>MMMASKDATSSVDGASGAGQLVPEVNASDPLAMDPVAGSSTAVATAGQVNPIDPWIINNFVQAPQGEFTISPNNTPGDVLFDLSLGPHLNPFLLHLSQMYNGWVGNMRVRIMLAGCAFTAGKIIVSCIPPGFGSHNLTIAQATLFPHVIADVRTLDPIEVPLEDVRNVLFHNNDRNQQTMRLVCMLYTPLRTCGGTGDSFVVAGRVMTCPSPDFNFLFLVPPTVEQKTRPFTLPNLPLSSLSNSRAPLPISSMGISPDNVQSVQFQNGRCTLDGRLVGTTPVSLSHVAKIRGTSNGTVINLTELDGTPFHPFEGPAPIGFPDLGGCDWHINMTQFGHSSQTQYDVDTTPDTFVPHLGSIQANGIGSGNYVGVLSWISPPSHPSGSQVDLWKIPNYGSSITEATHLAPSVYPPGFGEVLVFFMSKMPGPGAYNLPCLLPQEYISHLASEQAPTVGEAALLHYVDPDTGRNLGEFKAYPDGFLTCVPNGASSGPQQLPINGVFVFVSWVSRFYQLKPVGTASSARGRLGLRR[3x]

Noroviruses are single-stranded RNA viruses that cause pandemic outbreaks of acute gastroenteritis. Norovirus capsids are made of 180 identical copies of the VP1 protein arranged in a T = 3 icosahedral particle. The icosahedral asymmetric unit contains three quasi-equivalent VP1 monomers (designated A, B, and C). Each monomer associates with another monomer to form P domain dimers (in either A–B or C–C configuration).

The design of cysteine pairs within the shell domain of VP1 monomers can lead to the formation of intermolecular disulfide bonds between A–A and A–B monomers. This, in turn prevents the disassembly of the particle into VP1 dimers. Because of the symmetry of the norovirus VLPs, a cysteine pair introduced near the strict fivefold symmetry axes would yield disulfides between every A–A monomer pairs. The same cysteine pair at the strict threefold symmetry axes would yield disulfide bonds between every B–C monomer pair. DS1 VLPs showed the characteristic icosahedral symmetry with T = 3 arrangement. Clear densities for the formation of the interprotomer disulfide between Cys116 and Cys193 were visible around the fivefold and threefold symmetry axes. In summary, we successfully designed cysteine mutations in the GI.1 shell domain that resulted in interprotomer disulfides, stabilizing the entire capsid. The resulting particles showed increased thermal stability as evidenced by the appearance of a second melting transition at 75 °C compared to a single transition at 64 °C for the wild-type particles. The lower temperature transition corresponds to the unfolding of the P domain, while the higher temperature transition likely corresponds to the stabilized shell domain. In particular, stabilized VLPs elicited a more focused immune response toward accessible epitopes, and (in the absence of adjuvant) the development of blockade titers was much faster than immunization with wild-type particles.>[2x]MMYRAPKT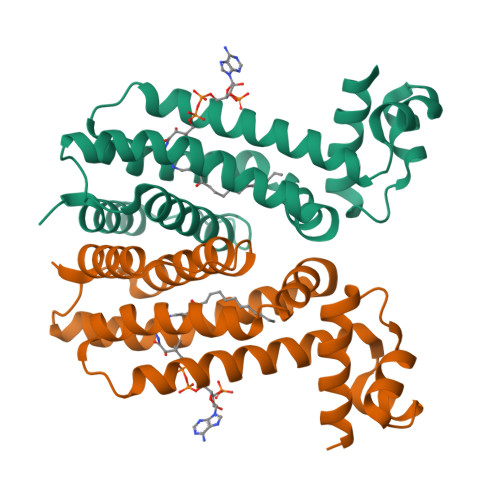EKGKESLNKILDASVELIADKGFLSTSINDITSKAGVAYGLFYFYFKSKHDILDEIIRQFNRNMRYYLKTYTQNLDSRIDVEKVGMKKFLEWMNENKKYYKIFIETQVHRPDIYKWHFMKLAERYTTGLSEAMRRGEIINVDPELLSYVLIGIAHMLGKRYVLWSNSGLTLKQQRDLDLIIENMLTPR>[3x]GMFIVNTNVPRASVPDGFLSE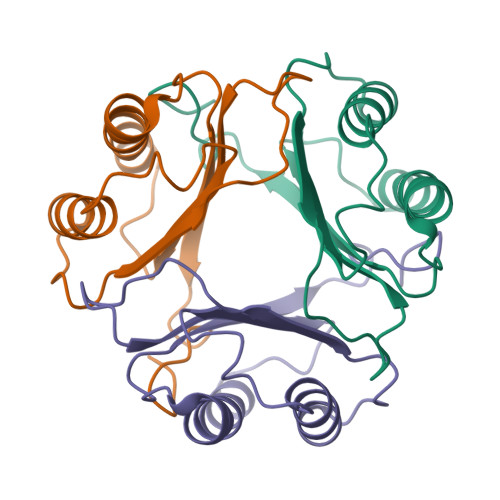LTQQLAQATGKPPQYIAVHVVPDQLMAFGGSSEPCALCSLHSIGKIGGAQNRSYSKLLCGLLAERLRISPDRVYINYYDMNAANVGWNNSTFA> GPLEDQEENTLRELRLFLRDVTKRLATDKRFNIFSKPVDIEEVSDYLEVIKEPMDLSTVITKIDKHNYLTAKDFLKDIDLICSNALEYNPDKDPGDKI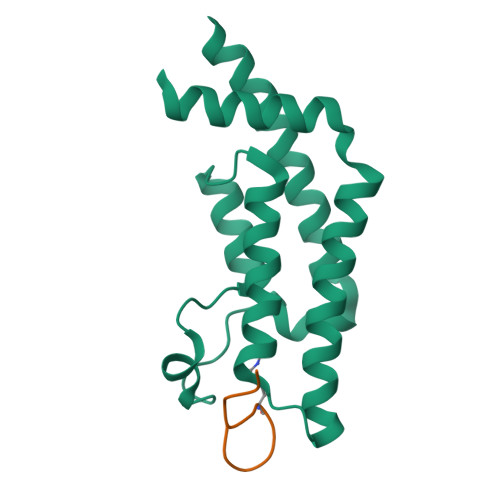IRHRACTLKDTAHAIIAAELDPEFNKLCEEIKEARIKR;>GKGGKGLGKGGAKR[2x]> TVDLNAFRLKSLAK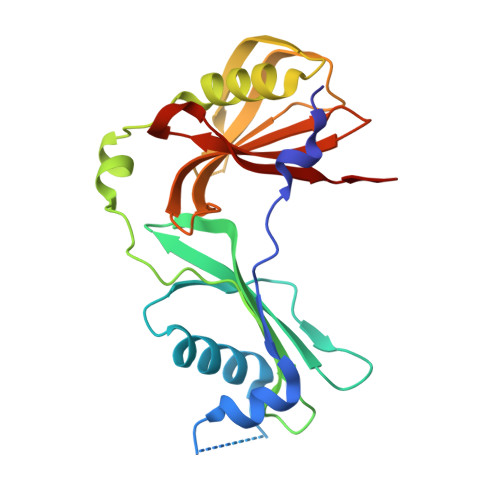YVNATETVIEAPSSFAPFKPQSYVEVATQHVKMIAPDATFRVVDDHYVGDNGVAHVHFRQTANGLDIDNADFNVNVGKDGKVFSYGNSFYTGQIPSSAALTKRDFSDPVTALKGTTNTLQLPITVDSASSESTEEKESYVFKGVSGTVSDPKAKLVYFVKDDGTLALAWRVETDIDSNWLLTYIDAKSGEEIHGVVDYVAE> GSLRQEDFPPRIVEHPSDLIVSKGEPATLNCKAEGRPTPTIEWYKGGERVETDKDDPRSH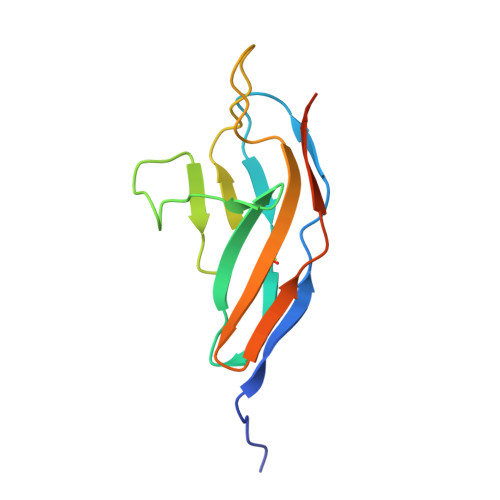RMLLPSGSLFFLRIVHGRKSRPDEGVYVCVARNYLGEAVSHDASLEVAAAAHHHHHH>[4x]PSTAGLGYGSWEIDPKDLTFLKELGTGQFGVV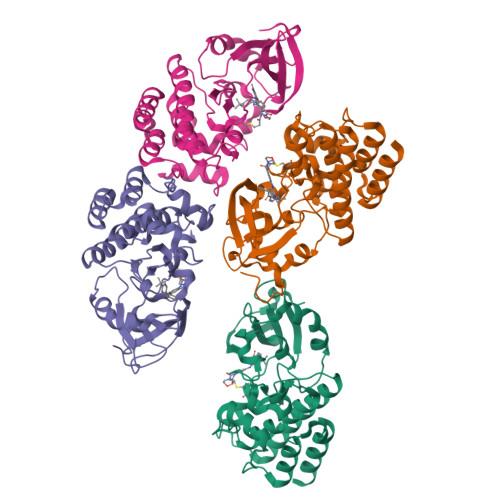KYGKWRGQYDVAIKMIKEGSMSEDEFIEEAKVMMNLSHEKLVQLYGVCTKQRPIFIITEYMANGCLLNYLREMRHRFQTQQLLEMCKDVCEAMEYLESKQFLHRDLAARNCLVNDQGVVKVSDFGLSRYVLDDEYTSSVGSKFPVRWSPPEVLMYSKFSSKSDIWAFGVLMWEIYSLGKMPYERFTNSETAEHIAQGLRLYRPHLASEKVYTIMYSCWHEKADERPTFKILLSNILDVMDEE> MHHHHHHMSWNHQSVEIAVRRTTVPSPNLPPGFDFTDPAIYAERLPVAEFAELRS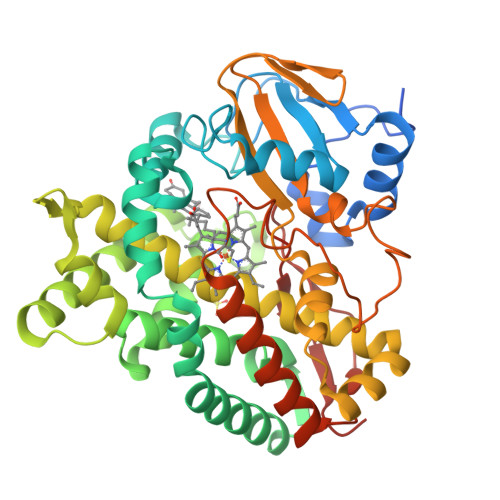AAPIWWNGQDPGKGGGFHDGGFWAITKLNDVKEISRHSDVFSSYENGVIPRFKNDIAREDIEVQRFVMLNMDAPHHTRLRKIISRGFTPRAVGRLHDELQERAQKIAAEAAAAGSGDFVEQVSCELPLQAIAGLLGVPQEDRGKLFHWSNEMTGNEDPEYAHIDPKASSAELIGYAMKMAEEKAKNPADDIVTQLIQADIDGEKLSDDEFGFFVVMLAVAGNETTRNSITQGMMAFAEHPDQWELYKKVRPETAADEIVRWATPVTAFQRTALRDYELSGVQIKKGQRVVMFYRSANFDEEVFQDPFTFNILRNPNPHVGFGGTGAHYCIGANLARMTINLIFNAVADHMPDLKPISAPERLRSGWLNGIKHWQVDYTGRCPVAH> IWELKKDVYVVELDWYPDAPGEMVVLTCDTPEEDGITWTL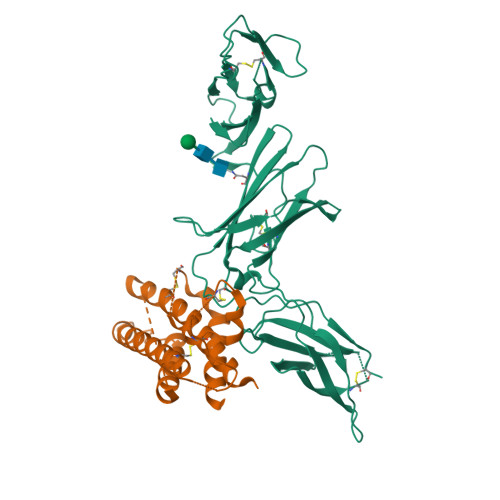DQSSEVLGSGKTLTIQVKEFGDAGQYTCHKGGEVLSHSLLLLHKKEDGIWSTDILKDQKEPKNKTFLRCEAKNYSGRFTCWWLTTISTDLTFSVKSSRGSSDPQGVTCGAATLSAERVRGDNKEYEYSVECQEDSACPAAEESLPIEVMVDAVHKLKYENYTSSFFIRDIIKPDPPKNLQLKPLKNSRQVEVSWEYPDTWSTPHSYFSLTFCVQVQGKSKREKKDRVFTDKTSATVICRKNASISVRAQDRYYSSSWSEWASVPCS;> RNLPVATPDPGMFPCLHHSQNLLRAVSNMLQKARQTLEFYPCTSEEIDHEDITKDKTSTVEACLPLELTKNESCLNSRETSFITNGSCLASRKTSFMMALCLSSIYEDLKMYQVEFKTMNAKLLMDPKRQIFLDQNMLAVIDELMQALNFNSETVPQKSSLEEPDFYKTKIKLCILLHAFRIRAVTIDRVMSYLNAS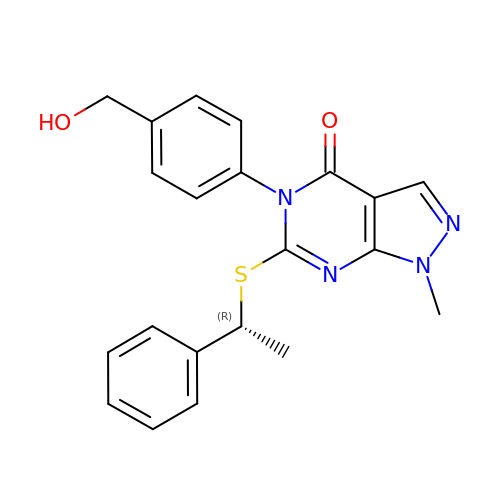5-[4-(hydroxymethyl)phenyl]-1-methyl-6-{[(1R)-1-phenylethyl]sulfanyl}-1,5-dihydro-4H-pyrazolo[3,4-d]pyrimidin-4-one | C21 H20 N4 O2 S | CXENUIKHQIZUDG-CQSZACIVSA-N> MQDSTSDLIPAPPLSKVPLQQNFQDNQFHGKWYVVGVAGNGFLREDKDPIKMAATIYELKEDKSYNVTFMKFPMKKCQYMTDTLVPGSQPGEF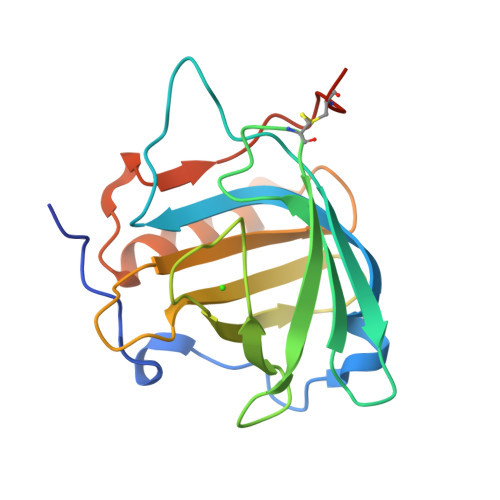TLGNIKSEPGYTSWLVRVVSTNYNQHAMVFFKAVQQNREDFFITLYGRTKELTSELKENFIRFSKSLGLPENHIVFPVPIDQCIDGSAHHHHHH> MKILLIGMGGTIASVKGENGYEASLSVKEVLDIAGIKDCEDCDFLDLKNVDSTLIQPEDWVDLAETLYKNVKKYDGIIVTHGTDTLAYTSSMISFMLRNPPIPIVFTGSMIPATEENSDAPLNLQTAIKFATSGIRGVYVAFNGKVMLGVRTSKVRTMSRDAFE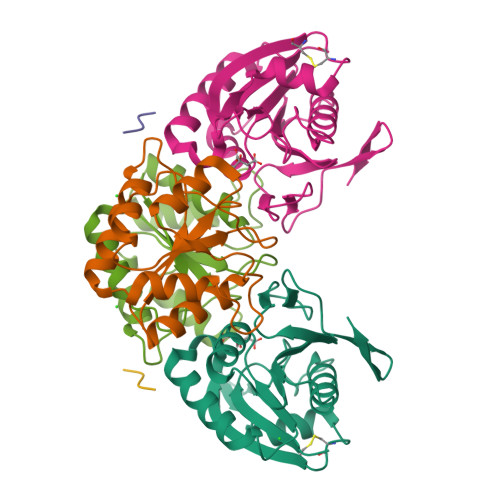SINYPIIAELRGEDLVVN;> MAVLVIKLIPGLSGDIFRAAVELGYRGIVIEGYGAGGIPYRGSDLLQTIEELSKEIPIVMTTQAMYDGVDLTRYKVGRLALRAGVIPAGDMTKEATVTKLMWILGHTNNVEEIKVLMRKNLVGELRD;> LVVN>[2x]MEKKEFH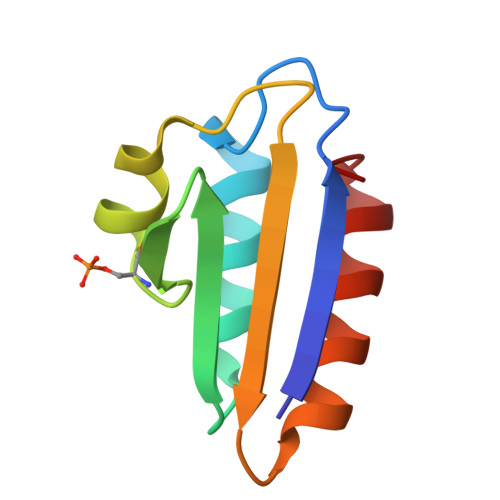IVAETGIHARPATLLVQTASKFNSDINLEYKGKSVNLKSIMGVMSLGVGQGSDVTITVDGADEAEGMAAIVETLQKEGLA> LTAKHRPSVVWLHNAECTGCTEAAIRTIKPYIDALILDTISL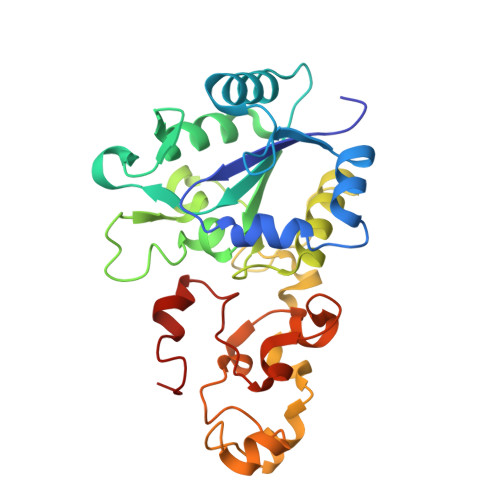DYQETIMAAAGETSEAALHEALEGKDGYYLVVEGGLPTIDGGQWGMVAGHPMIETCKKAAAKAKGIICIGTCSPYGGVQKAKPNPSQAKGVSEALGVKTINIPGCPPNPINFVGAVVHVLTKGIPDLDENGRPKLFYGELVHDNCPRLPHFEASEFAPSFDSEEAKKGFCLYELGCKGPVTYNNCPKVLFNQVNWPVQAGHPCLGCSEPDFWDTMTPFYEQG>[2x]GHHHHHHHHGSSTSNGMRCVGIGNRDFVEGLSGATWVDVVLEHGSCVTTMAKDKPTLDIELLKTEVTNPAVLRKLCIEAKISNTTTDSRCPTQGEATL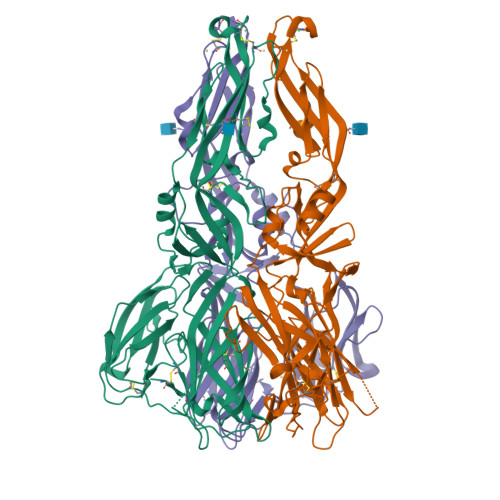VEEQDTNFVCRRTFVDRGHGNGCGLFGKGSLITCAKFKCVTKLEGKIVQYENLKYSVIVTVHTGDQHQVGNETTEHGTIATITPQAPTSEIQLTDYGALTLDCSPRTGLDFNEMVLLTMKEKSWLVHKQWFLDLPLPWTSGASTSQETWNRQDLLVTFKTAHAKKQEVVVLGSQEGAMHTALTGATEIQTSGTTTIFAGHLKCRLKMDKLTLKGMSYVMCTGSFKLEKEVAETQHGTVLVQVKYEGTDAPCKIPFSSQDEKGVTQNGRLITANPIVTDKEKPVNIEAEPPFGESYIVVGAGEKALKLSWFKKGSSIGKMFEATARGARRMAILGDTAWD> GPMVALSLKICVRHCNVVKTMQFEPSTAVYDACRVIRERVPEAQTGQASDYGLFLSDEDPRKGIWLEAGRTLDYYMLRNGDILEYKKKQRPQKIRMLDGSVKTVMVDDSKTVGELLVTICSRIGITNYEEYSLIQETIEEKKEEGTGTLKKDRTLLRDERKMEKLKAKLHTDDDLNWLDHSRTFREQGVDENETLLLRRKFFYSDQNVDSRDPVQLNLLYVQARDDILNGSHPVSFEKACEFGGFQAQIQFGPHVEHKHKPGFLDLKEFLPKEYIKQRGAEKRIFQEHKNCGEMSEI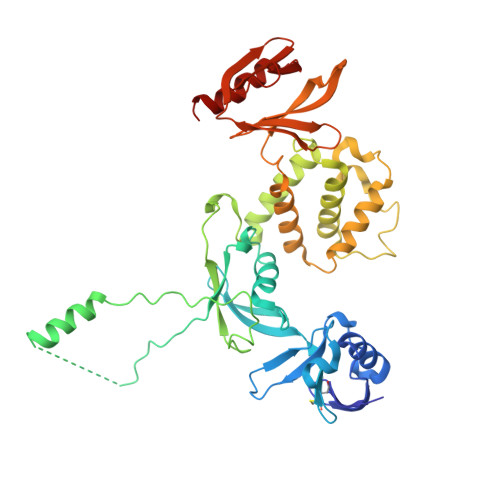EAKVKYVKLARSLRTYGVSFFLVKEKMKGKNKLVPRLLGITKDSVMRVDEKTKEVLQEWPLTTVKRWAASPKSFTLDFGEYQESYYSVQTTEGEQISQLIAGYIDIIL>[2x]AALADVILYEDDHILVLNKPSGTAVHGGSGLSFGVIEGLRALRPEARFL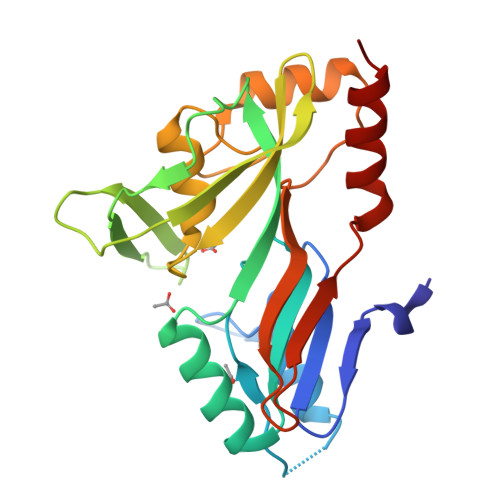ELVHRLDRDTSGVLLVAKKRSALRSLHEQLREKGMQKDYLALVRGQWQSHVKSVQAPLLKNILQSGERIVRVSQEGKPSETRFKVEERYAFATLVRCSPVTGRTHQIRVHTQYAGHPIAFDDRYGDREFDRQLTEAGTGLNRLFLHAAALKFTHPGTGEVMRIEAPMDEGLKRCLQKLRNAR The marine bacterium Salegentibacter sp. Hel_I_6 (Bacteroidota) isolated from seawater off Helgoland island (North Sea) contains an α-mannan inducible gene cluster with a GH76 family endo-α-1,6-mannanase (ShGH76). On overall, ShGH76 exhibited endo-α-1,6-mannanase activity with a preference for linear α-1,6-mannans. The tertiary structures of all three ShGH76 variants indicated a single-domain protein with a classical (α/α)6-barrel fold, with six α-helices forming a core that is surrounded by another six α-helices. Multiple sequence alignment identified the aspartates D136 and D137 as catalytic residues in ShGH76.

We solved the crystal structures of ShGH76WT (apo-form), ShGH76Asn (with Man3) and ShGH76Ala (with Man4) at 2.0 Å, 1.47 Å and 1.9 Å resolution, respectively. The ShGH76WT protein formed crystals belonging to the I 121 space group (Hermann-Mauguin notation) with three chains in an asymmetric unit (ASU), whereas the mutant protein ShGH76Ala crystallized in the P22121 space group with one chain in an ASU, and the mutant ShGH76Asn crystallized in the P1211 space group with one chain in an ASU. In the apo-form, in total twelve α-helices and six β-strands were present, whereas five β-strands were present in both substrate-bound mutant forms. The atomic models of the monomers of all three ShGH76 variants showed continuous peptide chains containing residues Asp54-Glu391. The ShGH76WT active site pocket is predominantly negatively charged - a trait that seems conserved based on surface electrostatic potential analyses with ConSurf. Besides negatively charged amino acids, the ShGH76 active site features seven aromatic amino acids (Trp90, Phe134, Trp140, Trp182, Phe256, Tyr258, Phe313). Superimposition of bound Man5 from BcGH76 suggests that Man5 does not fit the cavity of ShGH76WT due to a steric clash of the Trp254 of ShGH76WT. The terminal mannose of the Man3 and Man4 ligands adopted a kinked conformation so as to occupy the active site, which has not been shown in GH76 structures. Superimposition of ShGH76WT with ShGH76Ala and ShGH76Asn resulted in variations of 0.23 Å and 0.21 r.m.s.d, respectively, indicating minor loop movements on the protein surface but no global structural change as well as intact active site cores upon ligand binding.

>GSSHHHHHHSSGLVPRGSHMASSADDDGIDDVQEEEEEQPVEPGEEEDDEVADWGEVAENLQEQTYNIYLTSNGTFRQDNEGNENFNYWWNAHMLDVLIDGYERTGDESYLPKMKSLLEGIEVRNGNKYENVFIDDMEWLGIACLRTYKLTNDQQYKEVADLLWEETKQGWSDVHGGGIAWKTDTPNSKNACSNGPAAIFALYLYEIDQDEEDLEWAKKIYHWLKDTLVDPESGLVWDNIDYHDGEAIINRDWIFTYNVGTYIGAANLLHQATGEGMYLDDAIKSASSVVAPGELTTGGVLKNEGQGDGGLFKGILVRYFTQLALNPDLPDGKRNEFEEFVLFNAETLYHNGLTSAGLAGPNWNDEPSGRVDLSTQLSGVMLMEAKALLE[3x]We develop a hierarchical approach to designing multi-component protein assemblies from two classes of modular building blocks: designed helical repeat proteins (DHRs) and helical bundle oligomers (HBs). We first rigidly fuse DHRs to HBs to generate a large library of oligomeric building blocks. We then generate assemblies with cyclic, dihedral, and point group symmetries from these building blocks using architecture guided rigid helical fusion with new software named WORMS. X-ray crystallography and cryo-electron microscopy characterization show that the hierarchical design approach can accurately generate a wide range of assemblies, including a 43 nm diameter icosahedral nanocage.

The second protocol simplifies the process by overlapping the helical termini of the DHRs and HBs and designing only the immediate residues around the junction (HelixFuse, HF). For the second approach, HelixFuse (HF), the same set of DHRs and HBs were combinatorially fused together by overlapping the terminal helix residues in both directions (“AB”: c-terminus of HB to n-terminus of DHR, “BA”: n-terminus of HB to c-terminus of DHR). Sixteen tpr1C4_pm3 fusions were tested, 14 found to be soluble, and 10 displayed monodispersed peaks by SEC. C4_nat_HF-7900 was found to form monodisperse particles by cryo EM, with the 3D reconstruction modeled to 3.7 Å resolution. Inset shows the correct placement of the rotamers in the designed junction region. d C4_nat_HF-7900; design model (purple/grey) and cryo-EM map (yellow/white), with insert highlighting the the high resolution (~3.8 Å) density. e C5_HF-3921 as characterized by cryo-EM, with inset showing density surrounding the designed junction. f C5_HF-2101, g C5_HF-0019, h C6_HF-0075, and i C6_HF-0080 all showed a good overall match to its negative-stain EM 2D class averages (top) from one direction, using a predicted projection map (bottom). We show that it is possible to genetically fuse DHR “adapters” to natural proteins; these proteins can then be used in larger assemblies through WORMS with less likelihood of disrupting the original protein fold.

>ASSWVMLGLLLSLLNRLSLAAEAYKKAIELDPNDALAWLLLGSVLLLLGREEEAEEAARKAIELKPEMDSARRLEGIIELIRRAREAAERAQEAAERTGDPRVRELARELKRLAQEAAEEVRRDPDSKDVNEALKLIVEAIEAAVRALEAAERTGDPEVRELARELVRLAVEAAEEVQRNPSSSDVNEALKLIVEAIDAAVRALEAAEKTGDPEVRELARELVRLAVEAAEEVQRNPSSEEVNEALKDIVKAIQEAVESL[4x]> MSSVRAGVEAGRRDLTTFTFSGLQDAPVAALSGSIKLNVAAKAGKAEVTVAAGAAKAATQVSAAALRKL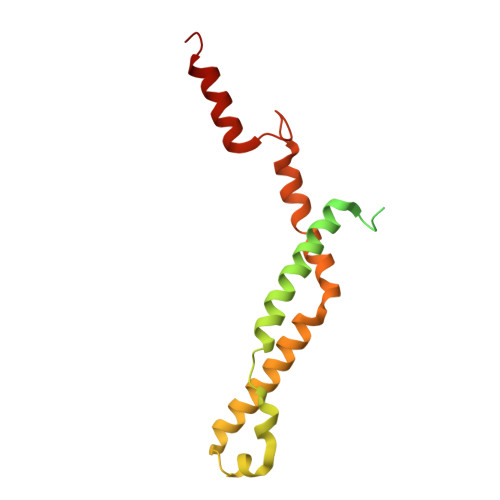SGSKISLAEVARISVLHSSIQNYLLSLSNERYQLLSQWPDFTTMYGKDFYYRAHPEDLKKFYDAADEYYKLYETVTEFDSLSALASQVVPNYAARRRSTVHPAIGSTVADGAFTNFLLSKQ> ESKKRQWALEDFEIGRPLGKGKFGNVYLAREKQSKFILALKVLFKAQLEKAGVEHQLRREVEIQSHLRHPNILRLYGYFHDATRVYLILEYAPLGTVYRELQKLSKFDE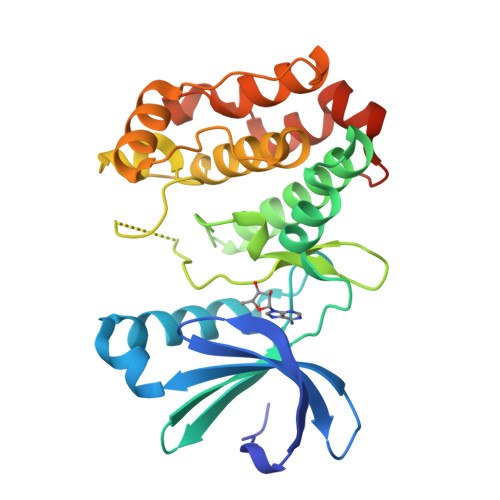QRTATYITELANALSYCHSKRVIYRDIKPENLLLGSAGELKIADFGWSVHAPSSRRTTLCGTLDYLPPEMIEGRMHDEKVDLWSLGVLCYEFLVGKPPFEANTYQETYKRISRVEFTFPDFVTEGARDLISRLLKHNPSQRPMLREVLEHPWITANSSKPSNCQNKESASKQS The human 8-oxoguanine DNA glycosylase 1 (hOGG1) is a bifunctional DNA repair enzyme that possesses both glycosylase and AP-lyase activity. Among DNA repair enzymes, human 8-oxoguanine glycosylase 1 (hOGG1) plays a central role in the base excision repair (BER) system acting against the strongly mutagenic 7,8-dihydro-8-oxoguanine (oxoG). To trigger the glycosylase reaction within a crystal, we created a pH-responsive mutant of hOGG1 in which lysine 249 (K249) has been replaced by histidine (H), and designated hOGG1(K249H). Thus, the hOGG1(K249H) mutant is a monofunctional enzyme with glycosylase activity alone.

As the hOGG1(K249H) mutant is almost inactive under basic conditions (pH >7.0), we crystallized the hOGG1(K249H)–DNA complex under weakly basic conditions (pH 8.0). In this way, we obtained a catalytically active hOGG1(K249H) mutant crystallized in a complex with an unreacted substrate, and determined the 3D structure of the pre-reaction ground state of the complex. The 3D structure of the complex was very similar to that determined by Vedine’s group. The oxoG base was flipped out from the DNA duplex and bound to the catalytic site of the enzyme. The H249 residue was located within the catalytic pocket, but the distance between Nϵ of H249 [Nϵ(H249)] and C1′ of oxoG [C1′(oxoG)] was 3.9 Å. The distance indicates that a direct nucleophilic attack of the Nϵ(H249) atom to the C1′(oxoG) atom is unlikely even if we consider a conformational change of the side chain in H249. On the other hand, a water molecule was found within a hydrogen-bonding distance from Nϵ(H249) and Oγ of S147 [Oγ(S147)], which may indicate the catalytic role of the water molecule. In the other catalytic residue, D268, one of its carboxy oxygen atoms is close to O4′(oxoG). In the ground-state structure of the hOGG1(K249H)–DNA complex, no proton-donating residue can access the N9(oxoG) site.

> GPGHRTLASTPALWASIPCPRSELRLDLVLPSGQSFRWREQSPAHWSGVLADQVWTLTQTEEQLHCTVYRGDKSQASRPTPDELEAVRKYFQLDVTLAQLYHHWGSVDSHFQEVAQKFQGVRLLRQDPIECLFSFICSSNNNIARITGMVERLCQAFGPRLIQLDDVTYHGFPSLQALAGPEVEAHLRKLGLGYRARYVSASARAILEEQGGLAWLQQLRESSYEEAHKALCILPGVGTHVADCICLMALDKPQAVPVDVHMWHIAQRDYSWHPTTSQAKGPSPQTNKELGNFFRSLWGPYAGWAQAVLFSADLRQSRHAQEPPAKRRKGSKGPEG>MRICLFLCLCLCMASPALAQVAVFPALSGKTDAQTLVVYSSLDEPLATPMIEGFQKANPDIAVHYEDMLTGEIYDRIVKETDAGKKTADFAFSSAMDLQVKLSNDGYAQRSDLAMSARWPAWANWRNTAYALTFEPAVFVYHKPSFTTEKPPATRAEFVDYLERHAKEVHGRIATYDIERSGVGFLFMSRDQEQFGDIWSVIKAMGAAGVKVYSTSSAILERVSDGRFVLGYNILGSYAADWASRH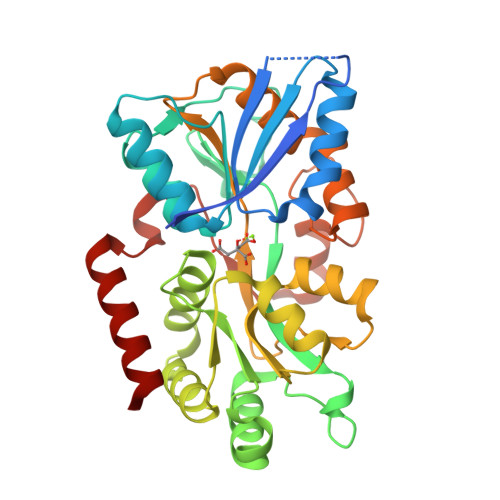PDVGIVLPKDYTVVMSRIGLVPEAAANPELGRRYLEFFMSKEGQTIMARQLQIPAVSPEVAGENTANTMQAIHGAQLRPVPVSPGLMVYLDQVKRSRLIERWNEALRSQ[2x]>[2x]HHHHHHSSGLVPRGSHMQTTTVYSLEDLLPYLKQDNVDVKLAPGTYNVNGFDVGEDRLFSTTPLFLFEGSNSTYDFTDVKLNINTVVLTKFGNNEVNEIQILGNNNVLKNLKLEDIGTTAPSNRAQSIVIDGRDNRIEGFHLTIRGSYPYGYGDAFGKGGGSVINHRKHSGVLIRGLRNHL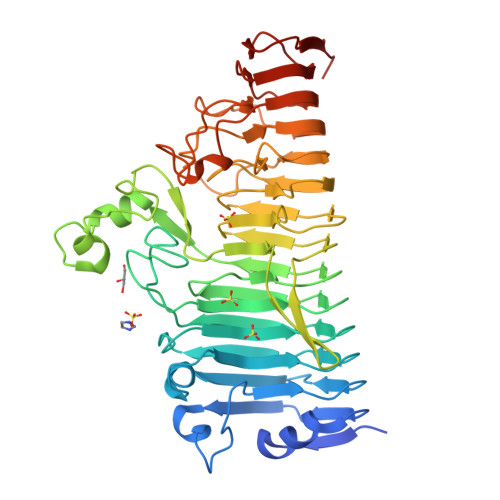KDCTIISRSYGHIVFMQAASYPTVEGCYIEGEMRSTDDMLAEEGTGSPADKVDFMTVWGYKLPAGYMMSLQEGGIRAYNAGTTYIDGVEIQRATDNPTVLNCTIKNARTGVTLAHANGTKYVEGCTVLGCENGYSIGSGTVVNCGADAIYGPVFKNTYGSDKGYNADITILPPSDAYYNGHDAVAYIGGSNHNLTFRSEITEIPSNLKIMVSGDLQGLRVLHGSNPSQNNFAGTNIVLRNLTNFPVDLHSDSSNITVTSCDTDNITDNGTNNSIEAIDCDSD The COMMD (Copper Metabolism Murr1 (Mouse U2af1-rs1 region 1) Domain) proteins are highly conserved in metazoans and unicellular protozoa. There are ten family members that play key roles in intracellular trafficking and in the regulation of transcription. A hallmark of the COMMD family members is a highly conserved C-terminal sequence of ~70–80 amino acids called the COMM domain, which has no known structure. The N-terminal domain of these proteins, which we refer to as the HN (helical N-terminal) domain, is more variable in sequence across the ten proteins, and is proposed to ascribe unique functions to the different family members.

We determined the crystal structure of the Commd9 COMM domain to 2.2 Å resolution by single-wavelength anomalous dispersion (SAD). The overall structure of the Commd9 COMM domain is composed of two cone-shaped chains that are tightly intertwined with each other to form a globular dimeric module. Each monomer is comprised of an N-terminal three-stranded β-sheet capped by an α-helix, with the overall arrangement making an open, hairpin-like structure. A simple analogy for the COMM domain dimer is that it resembles a left-handed handshake, where the sheet and helix from each monomer represent the interlocked palms and thumbs of each hand respectively. The overlapping C-terminal α-helices of each chain bury a large hydrophobic surface area of approximately 2100 Å2 (nearly 1/3rd of the monomer surface area) supporting the notion that the native state of COMMD proteins is to form dimers via the COMM domain. There is a very high degree of sequence conservation seen in the hydrophobic core of the Commd9 COMM domain, particularly along the α-helical surface mediating dimerisation. The high degree of conservation, and high degree of hydrophobicity within the dimerization interface strongly suggests that all of the COMMD proteins will form obligatory dimeric structures through similar mechanisms. We attempted to mutate several interfacial residues, but both the full-length mutated COMMD proteins and isolated COMM domains were aggregated due to poor protein solubility (not shown). This provides further support for the essential nature of dimer formation. The COMM domain fold is structurally related to the repeat domains found in the PUR (purine-rich element binding protein) family protein Pur-α.

>[2x]MANQISLPRLVDLDWRVDIKTSSDSISRMAVPTCLLQMKIQEDPSLCGDKPSISAVTVELSKETLDTMLDGLGRIRDQLSAVASKLEHHHHHH6-chloranyl-~{N}-(1-methylcyclopropyl)-1,1-bis(oxidanylidene)-4~{H}-thieno[3,2-e][1,2,4]thiadiazin-3-amine | C9 H10 Cl N3 O2 S2 | 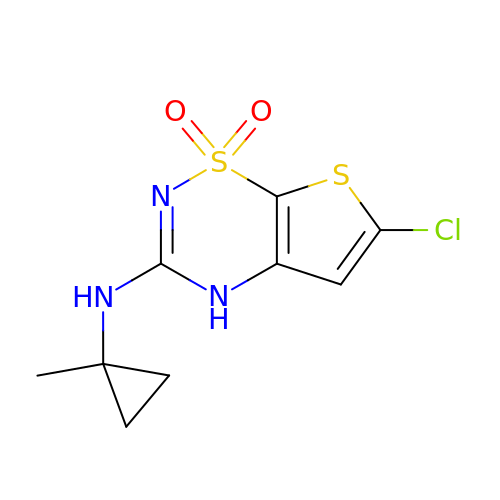KYSFUHHFTIGRJN-UHFFFAOYSA-N> TLPLWIGKPGDKPPPLCGAIPASGDYVARPGDKVAARVKAVDGDEQWILAEVVSYSHATNKYEVDDIDEEGKERHTLSRR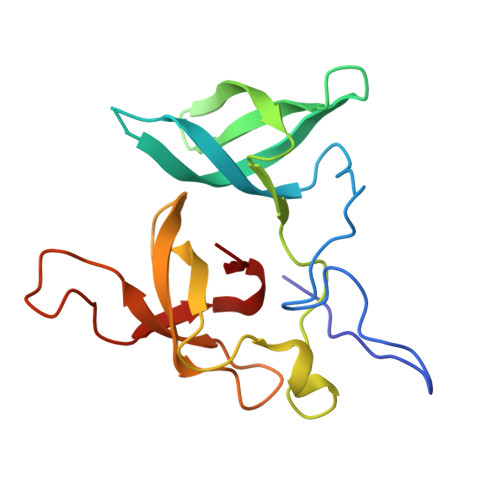RVIPLPQWKANPETDPEALFQKEQLVLALYPQTTCFYRALIHAPPQRPQDDYSVLFEDTSYADGYSPPLNVAQRYVVAC> GPMIDLYTAATPNGHKVSIALEEMGLPYTVHALSFDKKEQKAPEFLRINPNGRIPAIVDRSNDDFAVFESGAILVYLAEKTGQLMPTDVKGRSRVIQWLMFQMGGVGPMQGQANVFFRYFPEKLQGAIDRYQHETRRLYEVLDGRLGEAEYLAGDYSIADIATYPWVRIHDWSGVAVDGLDNLQRWIAALEARPAVQRGLLVPRREKEGDDAIR;> 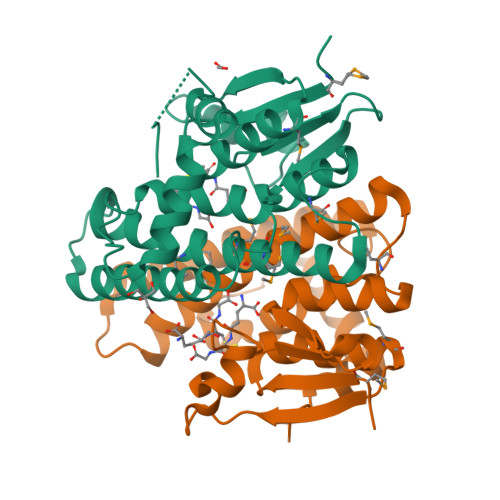GPMIDLYTAATPNGHKVSIALEEMGLPYTVHALSFDKKEQKAPEFLRINPNGRIPAIVDRSNDDFAVFESGAILVYLAEKTGQLMPTDVKGRSRVIQWLMFQMGGVGPMQGQANVFFRYFPEKLQGAIDRYQHETRRLYEVLDGRLGEAEYLAGDYSIADIATYPWVRIHDWSGVAVDGLDNLQRWIAALEARPAVQRGLLVPRREKEGDDAI;> GPMIDLYTAATPNGHKVSIALEEMGLPYTVHALSFDKKEQKAPEFLRINPNGRIPAIVDRSNDDFAVFESGAILVYLAEKTGQLMPTDVKGRSRVIQWLMFQMGGVGPMQGQANVFFRYFPEKLQGAIDRYQHETRRLYEVLDGRLGEAEYLAGDYSIADIATYPWVRIHDWSGVAVDGLDNLQRWIAALEARPAVQRGLLVPR;> PMIDLYTAATPNGHKVSIALEEMGLPYTVHALSFDKKEQKAPEFLRINPNGRIPAIVDRSNDDFAVFESGAILVYLAEKTGQLMPTDVKGRSRVIQWLMFQMGGVGPMQGQANVFFRYFPEKLQGAIDRYQHETRRLYEVLDGRLGEAEYLAGDYSIADIATYPWVRIHDWSGVAVDGLDNLQRWIAALEARPAVQRGLLVPR> GMINTKEDFLLLIKQIEQKSGYKKPKAFGIARLDRGQLNKNKILQASFALINYEQNFGSAAIMLEAFMQRGVEIDFNASEFVQTLKLEDIDFALSCFKPFLEEDGHQNIDLLKIIKDKFKDDEFSFVCLFEDKEPLSVESIYLKLYLLSTKKVPLRSINLNGAFGLLSNVAWSDDKPIELEYLRANEMRLKMSNQYPKIDFVDKFPRFLAHIIPEDNTRILESSKVRMGASLAAGTTIMPGASYVNFNAGTTGACMVEGRISS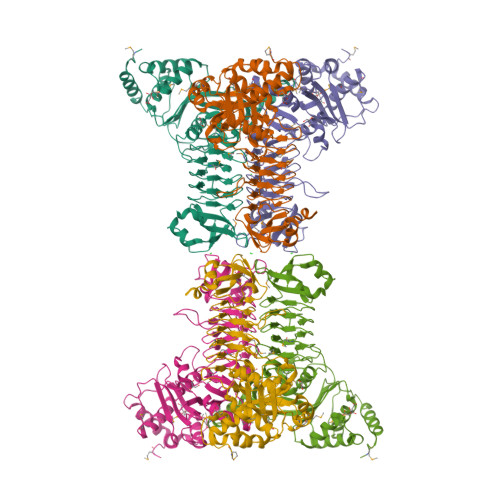SAIVGEGSDVGGGASILGVLSGTSGNAISVGKACLLGANSVTGIPLGDNCIVDAGIAVLEGTKFLLKDAEELAKLNPYFNFDKEIYKGLELKGLNGLHFRQDSISGAMIVALNKKAVKLNEALH>[3x]MALREDRIAEIVERVLARLGSGSGSGSG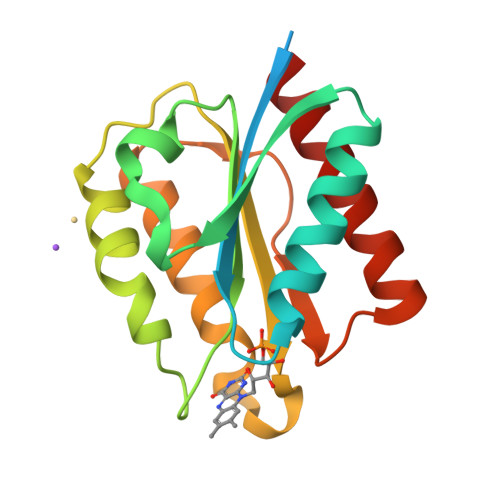SMLTAHVVYATMTGNNEEVANIVCDSLTNLNVKVTESEISQTDVADFMKADILVVCAYTYDEGAMPEEGLDFYDDLQSTDLTGKVYGVAGSGDKFYGEYFNTTVDHFDDAFKKAGATSGAEKVKIDLEPYEEDIERLNKFAEGLVKTASK>MASWSHPQFEKGALEDPRSLYDLPPYGDATLLYFSDLHGQAFPHYFMEPPNLIAPKPLMGRPGYLTGEAILRYYGVERGTPLAYLLSYVDFVELARTFGPIGGMGALTALIRDQKARVEAEGGKALVLDGGDTWTNSGLSLLTRGEAVVRWQNLVGVDHMVSHCEWTLGRERVEELLGLFRGEFLSYNIVDDLFGDPLFPAYRIHRVGPYALAVVGASYPYVKVSHPESFTEGLSFALDERRLQEAVDKARAEGANAVVLLSHNGMQLDAALAERIRGIDLILSGHTHDLTPRPWRVGKTWIVAGSAAGKALMRVDLKLWKGGIANLRVRVLPVLAEHLPKAEDVEAFLKAQLAPHQDHLFTPLAVSETLLYKRDTLYSTWDQLVGEAVKAIYPEVEVVFSPAVRWGTTILPGQAITWDHLYAYTGFTYPELYLFYLRGAQIKAVLEDIASNVFTSDPFYQQGGDVSRVFGLRYVL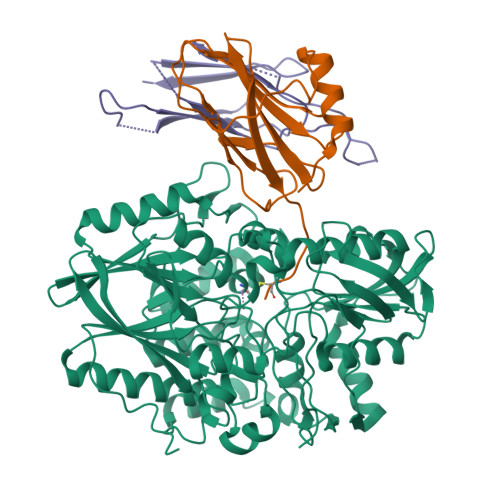DPDAPTGERVREVEVGGRPLDPNRRYLAAAYGGRLQRVGEAKPGYEPRPIYEVLAEYLRSVGRVRVRPEPNVKVIGRNYRLPEVTG[4x];>MRGSHHHHHHGSQGLEGEDLEHLEQALKEVFGKGFKDLTPSDAVKLNMPAIAESGANVPAEVEVALPKEQVRAIHLFADKNPTPHILAFMPMKAEPYYATRVRLAETTAIRAVVETQDGKLLLASASTRVTVGGCG[4x];>MPFRTIARLNPAKPKAGEEFRLQVVAQHPNEPGTRRDAEGKLIPAKYINLVEVYFEGEKVAEARPGPSTSANPLYAFKFKAEKAGTFTIKLKDTDGDTGEASVKLELA[4x]> APLNAARPAEERAALLAWVKERLHEEYGDQDPTPRRDPMHELISTILSQRTTHADEEAAYQELRTLGDWDAITLAPTDAVAHAIRRSNLPESKAPRIQETLRRIKAAPGGYDLDFLRDLPVKDALKWLTDLPGVGVKTASLVLLFNYARPVFPVDTHVHRVSTRVGVIPRMGEQAAHRALLALLPPDPPYLYELHINFLSHGRQVCTWTRPKCGKCILRERCDAYALYGDKVPSFSEKPVKGEKPAKG

Endonuclease III (EndoIII) is a ubiquitous bifunctional DNA glycosylase belonging to the helix-hairpin-helix (HhH)-GDP superfamily of DNA glycosylases. It is active for a broad range of oxidized pyrimidine lesions, removing numerous forms of modified thymine and cytosine bases from DNA, such as thymine glycol (Tg), a major stable oxidative modification of thymine, via the Base Excision Repair (BER) pathway. The crystal structures of EndoIIIs from E. coli (EcEndoIII) D. radiodurans (DrEndoIII1 and DrEndoIII3) and G. stearothermophilus (GsEndoIII) revealed that these enzymes comprise two domains divided by a positively charged DNA binding cleft containing the HhH motif and the catalytic residues Asp and Lys. D. radiodurans possesses three genes encoding EndoIII-like enzymes (DrEndoIII1, DrEndoIII2 and DrEndoIII3), while other bacteria typically possess one.

DrEndoIII1 displays a lower activity towards the common substrates and act mostly as a monofunctional DNA glycosylase. In DrEndoIII1 we substituted Arg61 and Tyr100 in DIL1 and DIL2 with the equivalent residues found in DrEndoIII2 (Glu and Leu). DrEndoIII1 Y100L shows more compromised activity when compared with wild-type and DrEndoIII1 R61Q. Our results demonstrate that the affinity of the DrEndoIII1 mutants for the substrates (with THF:G mispair and C:G pair) is reduced when compared with the wild-type enzyme. In the Y100L mutant it may be caused by a reduced steric fit of the Gln to the opposite strand of the flipped-out base compared to Tyr. MutY also possesses a Tyr residue in the same position as DrEndoIII1, thus it is possible that this residue in some HhH DNA glycosylases is optimized for stabilization of the substrate upon DNA binding. The crystal structures were determined and refined to resolutions of 1.38, 1.95 and 1.89 Å for DrEndoIII1 R61Q, DrEndoIII1 Y100L and DrEndoIII3 G250T/N251H, respectively. Additionally, the DrEndoIII1 R61Q and Y100L crystal structures include two magnesium ions, and the DrEndoIII3 G250T/N251H crystal structure has two chloride ions.> SNARLAYINPELAQEEKNKGNEYFKKGDYPTAMRHYNEA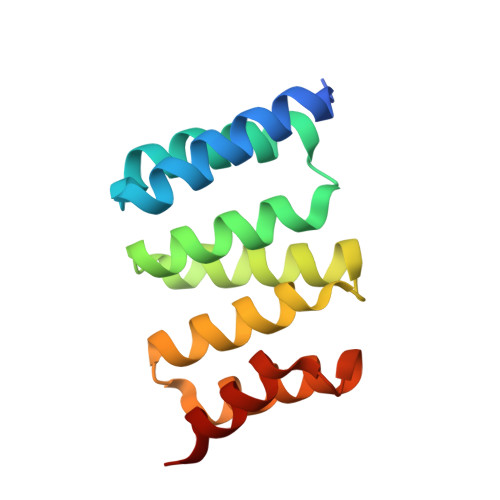VKRDPENAILYSNRAACLTKLMEFQRALDDCDTCIRLDSKFIKGYIRKAACLVAMREWSKAQRAYEDALQVDPSNEEAREGVRNCLR3-(1H-1,2,4-triazol-1-ylmethyl)aniline | C9 H10 N4 | 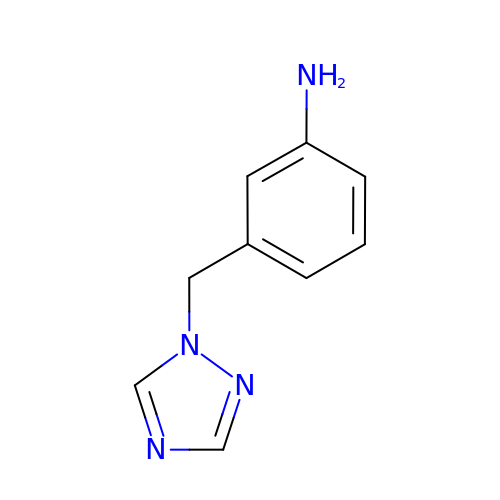LFINNEVQJQXPHN-UHFFFAOYSA-N(2Z,6Z,10Z,14Z,18Z,22E,26E)-3,7,11,15,19,23,27,31-octamethyldotriaconta-2,6,10,14,18,22,26,30-octaen-1-yl 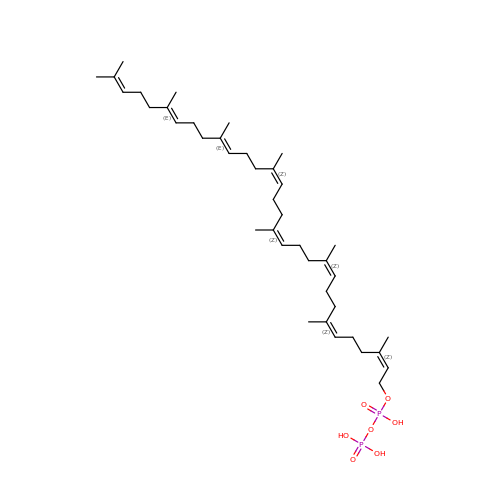trihydrogen diphosphate | C40 H68 O7 P2 | IKKLDISSULFFQO-MXWMMQQISA-N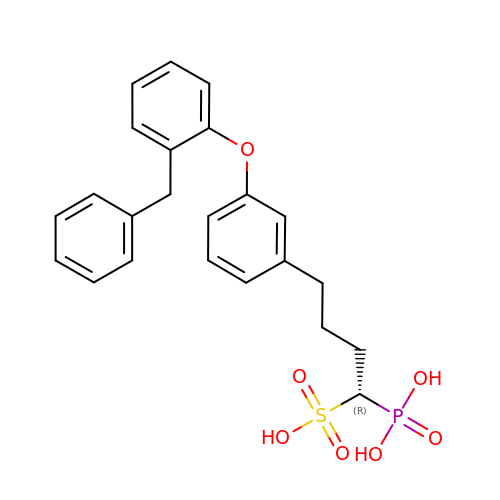(1R)-4-[3-(2-benzylphenoxy)phenyl]-1-phosphonobutane-1-sulfonic acid | C23 H25 O7 P S | ZMOCESLEEQXYRI-HSZRJFAPSA-N> MAYAQWVIIIIHNVGSQDVKIKN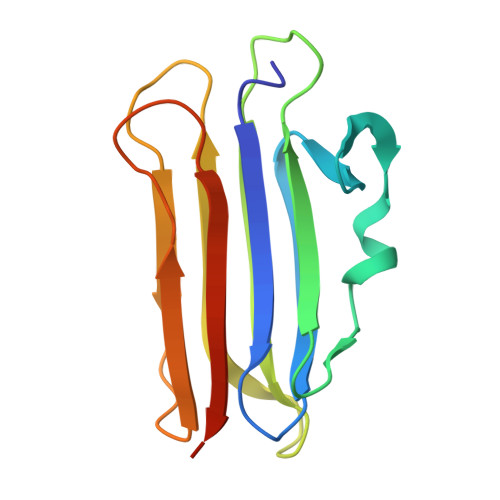LKASWGKLHADGDKDAEVSASNYEGKIVKPDEKLQINASGRSDAAEGTTGTFDLVDPADGDKQVRHFYWDSPWGSKTNTWTVSGSNTKWMIEYSGQNLDSGALGTITVDTLKKGENLYFQ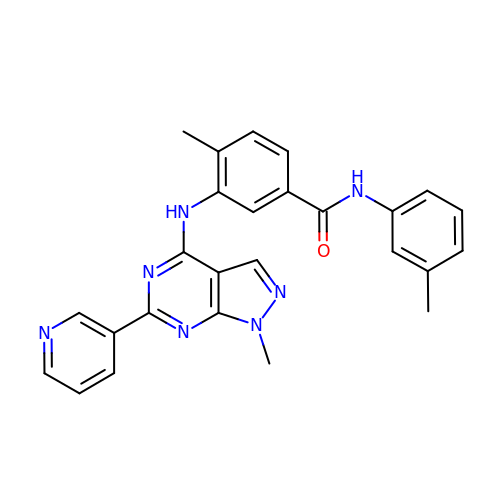4-methyl-~{N}-(3-methylphenyl)-3-[(1-methyl-6-pyridin-3-yl-pyrazolo[3,4-d]pyrimidin-4-yl)amino]benzamide | C26 H23 N7 O | BZJAAQAQRWJHJG-UHFFFAOYSA-N>[4x]MHHHHHHLEPPPSTFQPLCHPLVEEVSKEVDGYFLQHWNFPNEKARKKFVAAGFSRVTCLYFPKALDDRIHFACRLLTVLFLIDDLLEYMSFEEGSAYNEKLIPISRGDVLPDRSIPVEYIIYDLWESMRAHDREMADEILEPVFLFMRAQTDR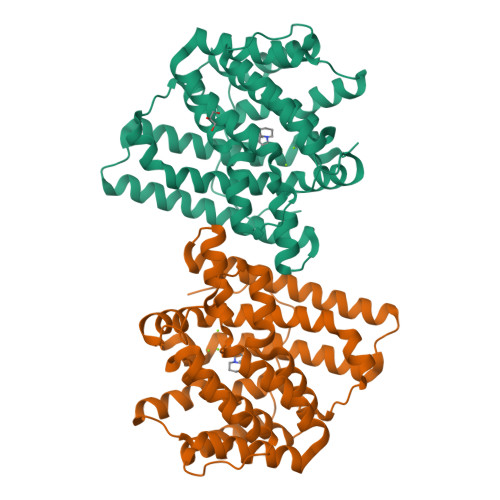TRARPMGLGGYLEYRERDVGKELLAALMRFSMGLKLSPSELQRVREIDANCSKHLSVVNDIYSYEKELYTSKTAHSEGGILCTSVQILAQEADVTAEAAKRVLFVMCREWELRHQLLVARLSAEGLETPGLAAYVEGLEYQMSGNELWAQTTLRYSVVVD> IPAGIIPTGNVLSTIEVCIFFRFLELGLSVACICTKFPELAYVRDGVIQFEVQQPMIARDGPHPVDQPVHNYMVKRIHKRSLSAAFAIASEALSLLSNTYVDGTEIDSSLRIRAIQQMARNLRTVSDSFERGTADQLLGVLLEKAPPLSLLSPINKFQPEGHLNRVARAALLSDLKRRVCADMFFMTRHAREPRLISAYLSDMVSCTQPSVMVSRITHTNTRGRQVDGVLVTTATLKRQLLQGILQIDDTAADVPVTYGEMVLQGTNLVTALVMGKAVRNARVPADLVIVGDKLVFLEALERRVYQATRVAYPLIGNIDITFIMPMGVFQANSMDRYTRHAGDFSTVSEQDPRQFPPQGIFFYNKDGILTQLTLRDAMGTICHSSLLDVEATLVALRQQHLDRQCYFGVYVAEGTEDTLDVQMGRFMETWADMMPHHPHWVNEHLTILQFIAPSNPRLRFELNPAFDFFVAPGDVDLPGPQRPPEAMPTVNATLRIINGNIPVPLCPISFRDCRGTQLGLGRHTMTPATIKAVKDTFEDRAYPTIFYMLEAVIHGNERNFCALLRLLTQCIRGYWEQSHR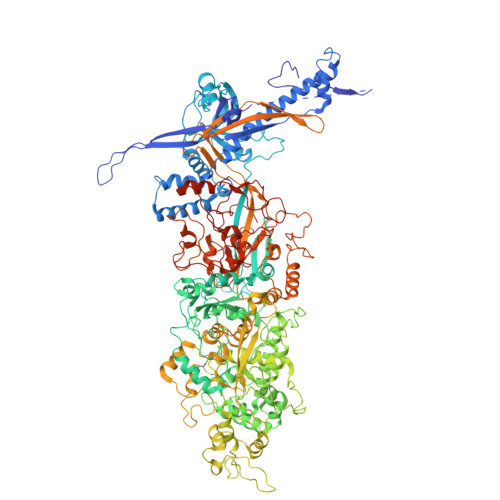VAFVNNFHMLMYITTYLGNGELPEVCINIYRDLLQHVRALRQTITDFTIQGEGHNGETSEALNNILTDDTFIAPILWDCDALIYRDEAARDRLPAIRVSGRNGYQALHFVDMAGHNFQRRDNVLIHGRPVRGDTGQAIPITPHHDREWGILSKIYYYIVIPAFSRGSCCTMGVRYDRLYPALQAVIVPEIPADEEAPTTPEDPRHPLHAHQLVPNSLNVYFHNAHLTVDGDALLTLQELMGDMAERTTAILVSSAPDAGAATATTRNMRIYDGALYHGLIMMAYQAYDETIATGTFFYPVPVNPLFACPEHLASLRGMTNARRVLAKMVPPIPPFLGANHHATIRQPVAYHVTHSKSDFNTLTYSLLGGYFKFTPISLTHQLRTGFHPGIAFTVVRQDRFATEQLLYAERASESYFVGQIQVHHHDAIGGVNFTLTQPRAHVDLGVGYTAVCATAALRCPLTDMGNTAQNLFFSRGGVPMLHDNVTESLRRITASGGRLNPTEPLPIFGGLRPATSAGIARGQASVCEFVAMPVSTDLQYFRTACNPRGRASGMLYMGDRDADIEAIMFDHTQSDVAYTDRATLNPWASQKHSYGDRLYNGTYNLTGASPIYSPCFKFFTPAEVNTNCNTLDRLLMEAKAVASQSSTDTEYQFKRPPGSTEMTQDPCGLFQEAYPPLCSSDAAMLRTAHAGETGADEVHLAQYLIRDASPLRGCLPL>[2x]XGEIAQALKEIAKALKEIAWALKEAAQALKGX

αHBs are oligomers of 5 or more α-helical peptides that assemble into coiled-coil structures with central solvent-accessible channels. We targeted two properties of αHBs: oligomeric state, which directly affects the internal diameter of the channel; and the identities of channel-facing residues, which fine tune this dimension and introduce different chemistries. The αHBs are loaded with an environment sensitive dye (in this case, 1,6-diphenyl-1,3,5-hexatriene, DPH) that binds within the channels and fluoresces. Accordingly, challenging the array with analytes leads to differential displacement of the dye across the array to give a fluorescent fingerprint.

Despite the requirements for aliphatic residues at a and d, up to 40% of these can be changed to other side chains without compromising barrel integrity. We introduced mutations at one or two of these sites to generate four groups of αHB: Group I had entirely hydrophobic interiors, but with different sizes and shapes of channel; Groups II and III had polar uncharged or polar charged residues, respectively, at specific points along the channel; and Group IV had aromatic residues installed in their channels. In detail, the sixteen Group I peptides included: previous designs for a pentamer, 3 hexamers, 2 heptamers and an octamer all verified by X-ray crystallography;27,29 single and/or double mutations to Ala and Gly at central a and d sites to generate larger channels; a single-Pro mutant at the final d site to kink and open the C-terminal end of the channel; and a variant with all a sites made Met to vary the hydrophobic chemistry used. Finally, one third of the designs were crystallized and yielded 12 X-ray crystal structures, all of which were open αHBs with fully accessible channels. Conversely, the FAs generate signal through interactions with the more-hydrophobic and aromatic-containing channels (Group I and IV).>[2x]MTKRLFLPEWAPQEAVQLTWPHDRTDWAYMLD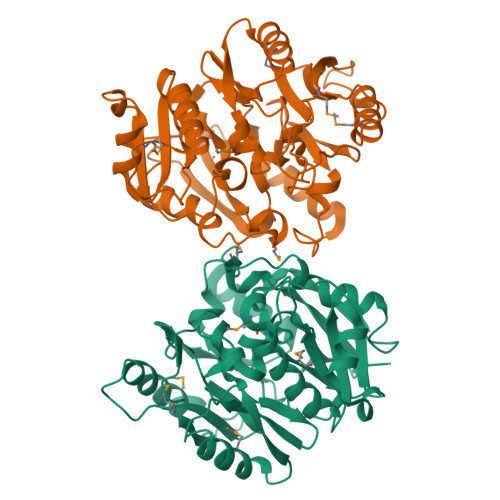EVETCFVRIATAILRHERLIVVCPDRKRVFGLLPPELHHRLYCFELPSNDTWARDHGGISLLADGRPMIADFAFNGWGMKFAAHHDNLITRRLHALGLFAEGVTLDNRLAFVLEGGALETDGEGTLLTTDSCLFEPNRNAGLSRTAIIDTLKESLGVSRVLSLRHGALAGDDTDGHIDTLARFVDTRTIVYVRSEDPSDEHYSDLTAMEQELKELRRPDGQPYRLVPLPMAEALYDGADRLPATYANFLIINGAVLVPTYDSHLDAVALSVMQGLFPDREVIGIDCRPLVKQHGSLHCVTMQYPQGFIRLEHHHHHH>[2x]NIGSQWRDDEVHFNRTLDSILVPRVVGSRGHQQVREYLVQSLNGLGFQTEVDEFKQRVPVFGELTFANVVGTINPQAQNFLALACHYDSKYFPNDPGFVGATDSAVPCAILLNTAKTLGAYLQKEFRNRSDVGLMLIFF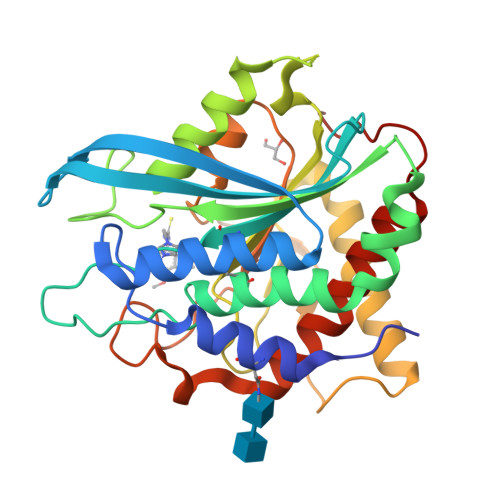DGEEAFKEWTDADSVYGSKHLAAKLASKRSGSQAQLAPRNIDRIEVLVLLDLIGARNPKFSSFYENTDGLHSSLVQIEKSLRTAGQLEGNNNMFLSRVSGGLVDDDHRPFLDENVPVLHLVATPFPDVWHTPRDNAANLHWPSIRNFNRVFRNFVYQYLKRHTSPVNLRFYRT>[3x]KPIEIIGAPFSKGQPRGGVEKGPAALRKAGLVEKLKETEYNVRDHGDLAFVDVPNDSPFQ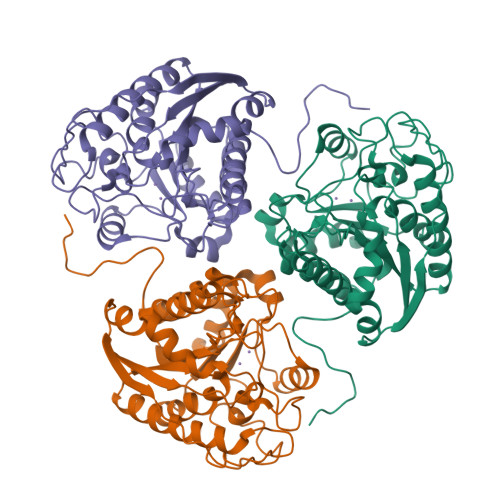IVKNPRSVGKANEQLAAVVAETQKNGTISVVLGGDHSMAIGSISGHARVHPDLCVIWVDAHTDINTPLTTSSGNLNGQPVAFLLKELKGKFPDVPGFSWVTPCISAKDIVYIGLRDVDPGEHYIIKTLGIKYFSMTEVDKLGIGKVMEETFSYLLGRKKRPIHLSFDVDGLDPVFTPATGTPVVGGLSYREGLYITEEIYKTGLLSGLDIMEVNPTLGKTPEEVTRTVNTAVALTLSCFGTKREGNHKPETDYL> MLGIVQKTATEQLDYDIDFARWMPDGDVLQSAGVVITPDDGTLTSPAYEIDGTVVKVWL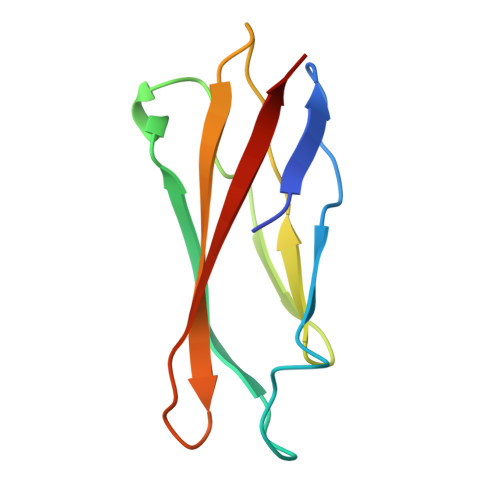AGGTAGASYNVDVTVATAAGRIKETCFKTRVRSC>[2x]GHMPNFSGNWKIIRSENFEELLKVLGVNVMLRKIAVAAASKPAVEIKQEGDTFYIKTSTTVRTTEINFKVGEEFEEQTVDGRPCKSLVKWESENKMVCEQ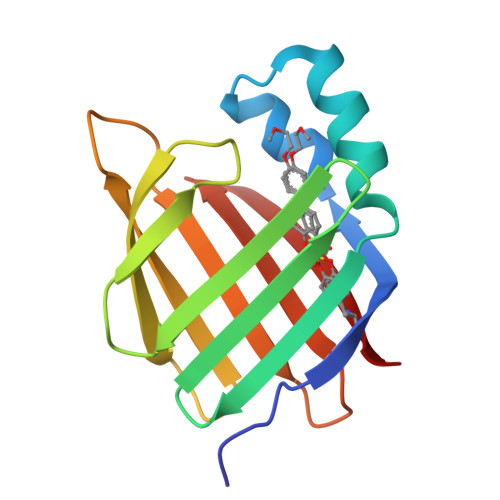KLLKGEGPKTSWTRELTNDGELILTMTADDVVCTRVYVRE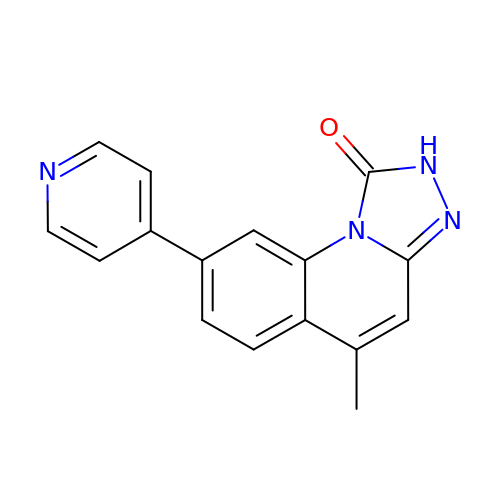5-METHYL-8-PYRIDIN-4-YL[1,2,4]TRIAZOLO[4,3-A]QUINOLIN-1(2H)-ONE | C16 H12 N4 O | PKZCGWBROCHAKF-UHFFFAOYSA-N> M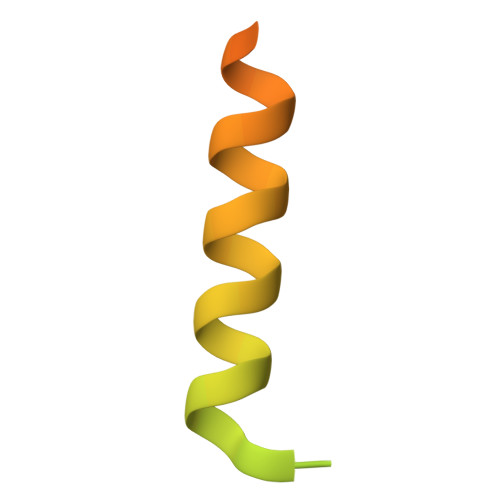KESKVPSSTDMEGKLKENQNENIKGHEAKKAHKPPPEDYEIWKARMLAKAQAKLKELEASQSHMDSQLLEA>[4x]MIKIPKRYLETEPYRIVENNFHPDKSMVSESIFSLGNEYSGTRAFFDETYSGKQLIGTYFNGIYEYALKDTPSAYLGIVKRTHFTINSVNFFKIRIIHEDEELDLNKVKFEDFKRILDLRSGLYQRTFTWLTNQAKIKIIISRLLDMSDCENAYQMISFESDIDTDIKLELHLDSNILHWGSDCYWNRVKEFKIGNSIGLTVKTLTTNQTLTSVMRTNLKEDSYQLNQKEVILNYELTLEANKEKTITRYVTNIIDKNGNQKL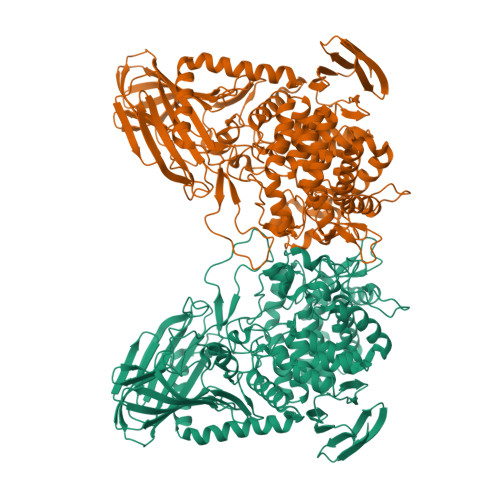SQQRDIALTKLKEASKFSFADLVKKNQKFFNHFYQKSDILIDGSDSDQQGIRYCLFQMIQAYHGFDPTNTIGAKGLTGEAYSGHAFWDNETYCLPFYLYSNQEAAKDLIMFRYNTLEEAKARAKELDSIGACFPVATRNGKEACNLWQHASTQFQPSTGVFYAIYHYMKIYNDHKFMQNYGIEMLVEISKFLLSRGQYNQDKTKFSFYGVMGPDEFKLMVNHNTYTNFMAKKCFQYLDKILADKTYKTDKILDKCGFTKKDLAKMKDASRKMVILYDKETLLFEQNDGFFDMPHVDIKTIKDEEMPIYSHWSYDRIYRTDIIKQPDVLMFMFLYMEEFSQKQLLANYNYYEPRTLHESSLSPSIHSIIASKIGLEKDANNFFGFATRLDLDDYNNNTCEGIHMTSIAAAWMNIVYGFGGLMIKNDILNLTPTSNKNWNYYQFKITFKNHLLTVKVDKDNVIITKKTKNILPINVYGKKYELIDKLEIKRAAENLYFQ> ATHTAQTQTHLNFTQIKTVDELNQALVEAKGKPVMLDLYADWCVACKEFEKYTFSDPQ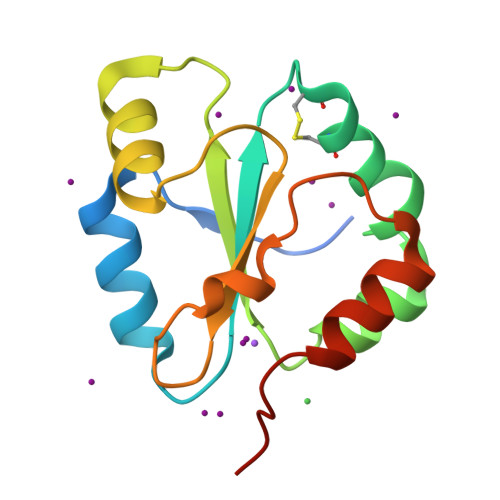VQKALADTVLLQANVTANDAQDVALLKHLNVLGLPTILFFDGQGQEHPQARVTGFMDAETFSAHLRDRQPHHHHHH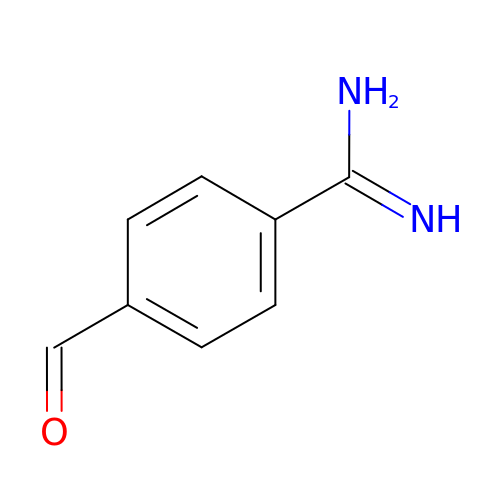4-formylbenzenecarboximidamide | C8 H8 N2 O | WMFQLLSIPXELTN-UHFFFAOYSA-N>GSHMKNSVSVDLPGSMKVLVSKSSNADGKYDLIATVDALELSGTSDKNNGSGVLEGVKADASKVKLTISDDLGQTTLEVFKSDGSTLVSKKVTSKDKSSTHEKFNEKGELSEKHITRADKSSTHEKFNEKGELSEKHITRADKSSTHEKFNEKGELSEKHITRADKSSTHEKFNEKGEVSEKHITRADGTRLEYTGIKSDGSGKAKEVLKGYVLEGTLTAEKTTLVVKEGTVTLSKNISKSGEVSVELNDTDSSAATKKTAAWNSGTSTLTITVNSKKTKDLVFTSSNTITVQQYDSNGTSL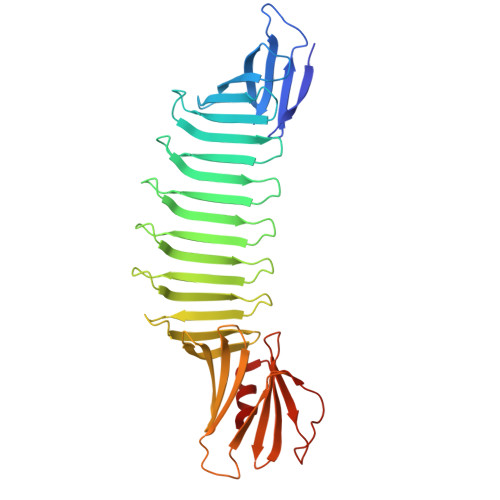EGSAVEITKLDEIKNALK[2x]> DETGVMDSLLEALQSGAAF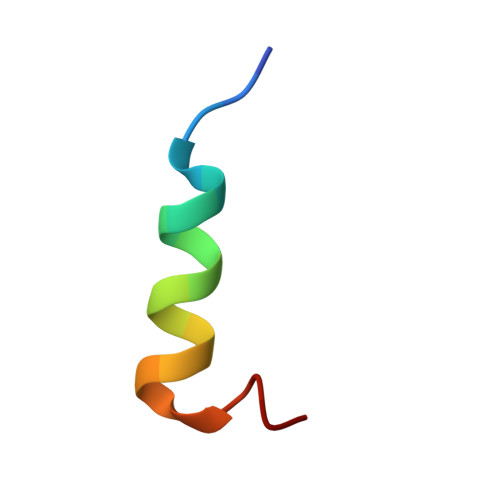R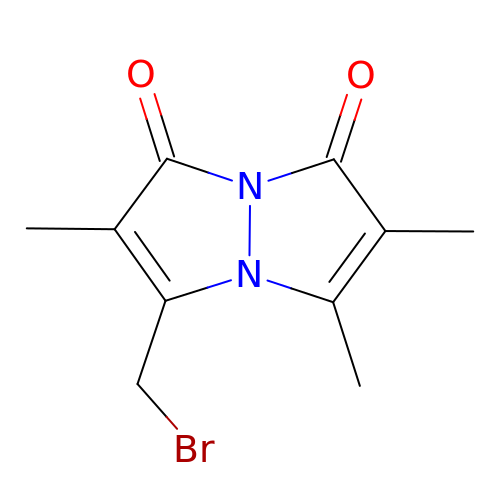3-(bromomethyl)-2,5,6-trimethyl-1H,7H-pyrazolo[1,2-a]pyrazole-1,7-dione | C10 H11 Br N2 O2 | AHEWZZJEDQVLOP-UHFFFAOYSA-N> FTD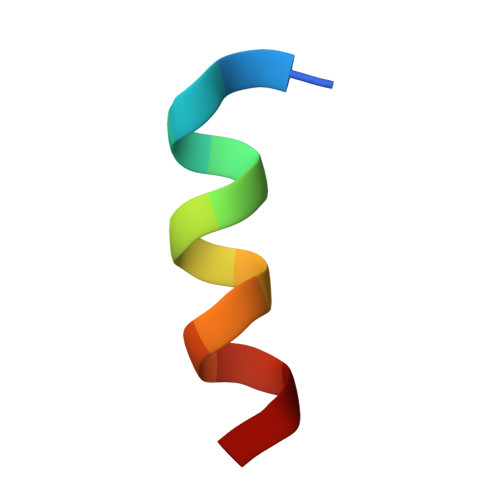CQLAAAVCMTY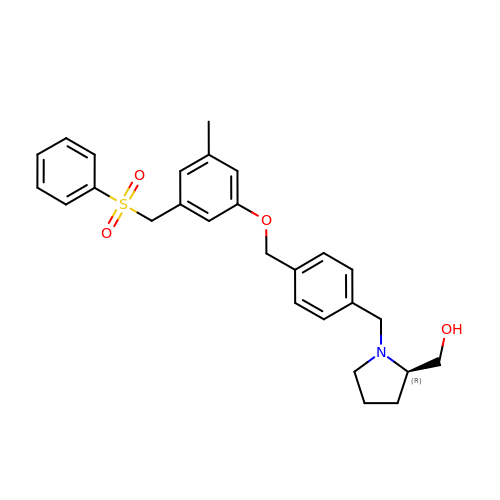{(2R)-1-[4-({3-METHYL-5-[(PHENYLSULFONYL)METHYL]PHENOXY}METHYL)BENZYL]PYRROLIDIN-2-YL}METHANOL | C27 H31 N O4 S | NPUXORBZRBIOMQ-RUZDIDTESA-N> MGGSSHHHHHHSSGLVPRGSGGLTHRKFGGSGGSPFSGLSSIAVRSGSALDAIIIDGVHHGGSGGNLSPTFTFGSGEYISNMTIRSGDYIDNISFETNMGRRFGPYGGSGGSANTLSNVKVIQINGSAGDYLDSLDI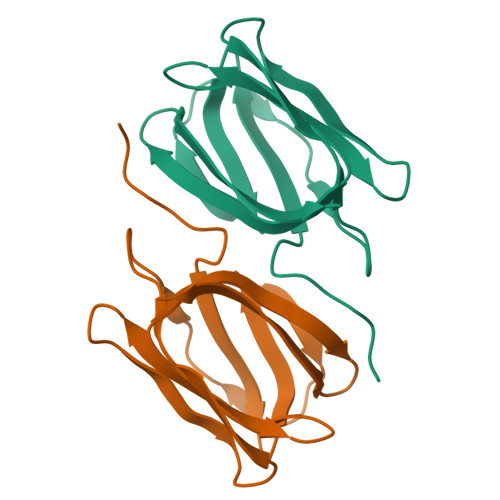YYEQY>LTGQIIEYTIKIQTIYTGNFKHKNGFLKMIERGIAMKKENLKILAKKAQTIAIVGANYRFATRVLLENLDKMDFTGTIYLVNPRYENIDGVRCYQSLLEIEDTIDVVVGLVNPQLMIQVASNASKINAKVLVIPGGGYGESGVEGQNIQNAILERAADSGMRIVGPNCMGYLNMHAQFTPYIGTLHRPLRPIKKGPVSIISQSGSVNDAFIASKLGISKIYSTGNEADVQMHDYLNLLAEDPETSVIILYIEAIRNHLSFLRALDLCSKNKKPVIAIKVGRTIKSAAVANAHSGALAGDYEIEKLFLEGHGVLFVEDIDQAVAVALLLSQPYLPTVNTVAALTVSGGQAGILLDLAEDYGVDFPDFSAVTNYEIASKLPELGGLSNPLDIWGKSSKDFSEVSNICLSSIVKDADIGIITVAIDAPIGQGDHEFDFTSIPAKDLASLRGNSDKPFLYFSHIQTEFDPRVESILDEAGIAVIQGSRNALVACRALFKYKEFLEKNNHTPIYSVEDL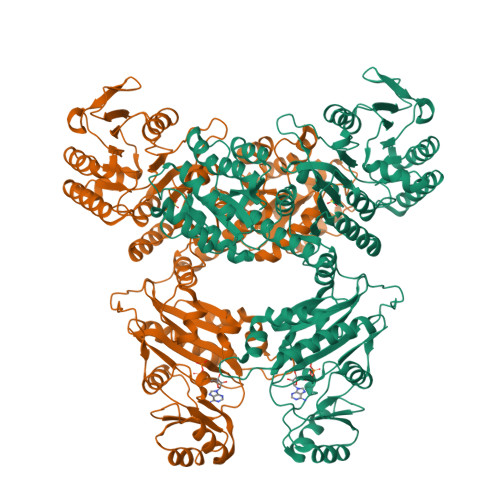SIQKGLKLLHDNEGRKLLDESGFVSPREQVVTSLQEGVDYAESIGYPVVLKAQGLAHKTDVGGVALNIKSAAKLKKAWGKMEHLNSPYYLIQEMVTDGFETILAYRTDMNYGPVVIFGLGGIYTELFNEVVLAVPPITHKKAEQMVKSIPMLWKSIEGYRGNPALDLEALTASIVQMGETAMEKYEEIVEFEINPLSVRVKGVVALDVLASVKTTAAKEADAEEADVKKCSELV[4x]> TPEMPVLENRAAQGDITAPGGARRLTGDQTAALRDSLSDKPAKNIILLIGDGMGDSEITAARNYAEGAGGFFKGIDALPLTGQYTHYALNKKTGKPDYVTDLAASATAWSTGVKTYNGALGVDIHEKDHPTILEMAKAAGLATGNVSTAELQDATPAALVAHVTSRKCYGPSATSEKCPG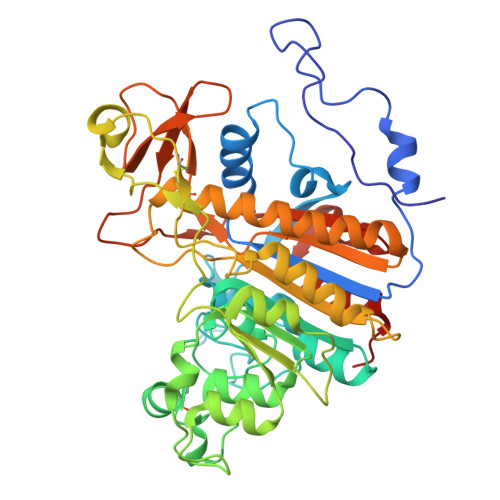NALEKGGKGSITEQLLNARADVTLGGGAKTFAETATAGEWQGKTLREQAQARGYQLVSDAASLNSVTEANQQKPLLGLFADGNMPVRWLGPKATYHGNIDKPAVTCTPNPQRNDSVPTLAQMTDKAIELLSKNEKGFFLQVEGASIDKQDHAANPCGQIGETVDLDEAVQRALEFAKKEGNTLVIVTADHAHASQIVAPDTKAPGLTQALNTKDGAVMVMSYGNSEEDSQEHTGSQLRIAAYGPHAANVVGLTDQTDLFYTMKAALGLKHHHHHH Here we identified 2′-phosphouridine (Up) at position 47 of tRNAs from thermophilic archaea. Up47 confers thermal stability and nuclease resistance to tRNAs. In addition, we identified the arkI gene, which encodes an archaeal RNA kinase responsible for Up47 formation. Taken together, our findings show that Up47 is a reversible RNA modification mediated by ArkI and KptA that fine-tunes the structural rigidity of tRNAs under extreme environmental conditions.

To this end, we treated S. tokodaii tRNAVal3 with yeast Tpt1p (2′-phosphotransferase) to remove the 2′-phosphate of Up47. To further investigate the structural role of Up47, we also solved a crystal structure for Tpt1p-treated S. tokodaii tRNAVal3. Both molecules A and B of the Tpt1p-treated tRNA showed the canonical structure with the standard core. In both molecules, U47 was dissociated from the s4U8– A14–A21 base triple with backbone angles α, γ and ε altered by 153°, –109° and –37°, respectively (molecule A), thereby placing the uracil base of U47 outwards. In another aspect of the Tpt1p-treated tRNA, C9 was detached from the C12–G23–C9 base triple in both molecules. Because the Tpt1p-treated tRNA has the canonical structure with the standard core, it is likely that the structural alteration is caused by Up47.

>[2x]GGGCCNGUCGUCUAXCCUGGUUAGGACGCCGCCCUUACAAGGCGGAGGUCCUGGGUUCGAGUCCCAGCGGGCCCACCA>[2x]ATLHSFVLVDNGGTGNVTVVPVSNANGVAEWLSNNSRSQAYRVTASYRASGADKRKYTIKLEVPKIVTQVVNGVELPVSAWKAYASIDLTIPIFAATDDVTVISKSLTGLFKVGNPIA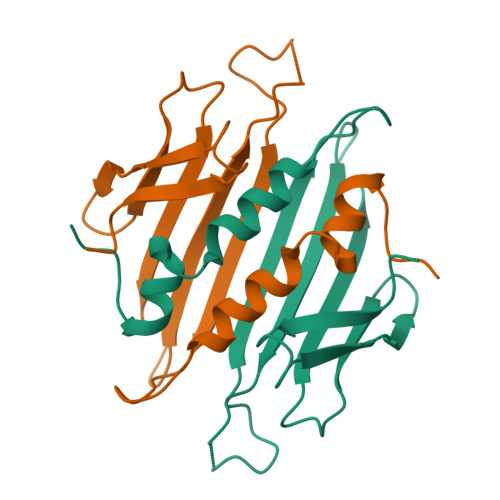EAISSQSGFYA> 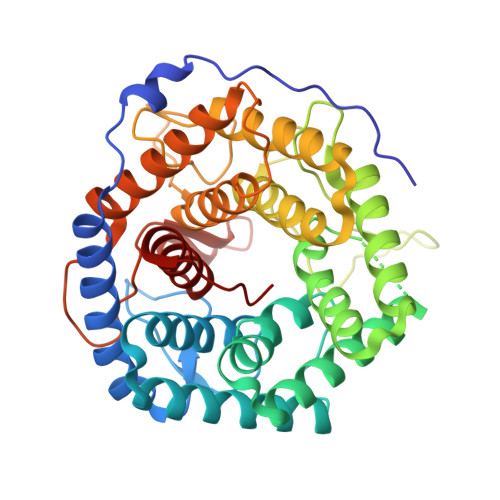MMKIKPVKVESIENPKRFLNSRLLTKIEVEEAIEKALKQLYINIDYFGEEYPTPATFNNIYKVMDNTEWTNGFWTGCLWLAYEYNQDKKLKNIAHKNVLSFLNRINNRIALDHHDLGFLYTPSCTAEYRINGDVKALEATIKAADKLMERYQEKGGFIQAWGELGYKEHYRLIINCLLNIQLLFFAYEQTGDEKYRQVAVNHFYASANNVVRDDSSAFHTFYFDPETGEPLKGVTRQGYSDESSWARGQAWGIYGIPLSYRKMKDYQQIILFKGMTNYFLNRLPEDKVSYWDLIFTDGSGQPRDTSATATAVCGIHEMLKYLPEVDPDKETYKYAMHTMLRSLIEQYSNNELIAGRPLLLHGVYSWHSGKGVDEGNIWGDYYYLEALIRFYKDWELYW> RLYRADSRPPDEIKRSGGLMPRGHNEYFDRGTQMNINLYDHARGTQTGFVRYDDGYVSTSLSLRSAHLAGQSILSGYSTYYIYVIATAPNMFNVNDVLGVYSPHPYEQEVSALGGIPYSQIYGWYRVNFGVIDERLHRNREYRDRYYRNLNIAPAEDGYRLAGFPPDHQAWREEPWIHHAPQGCG;> GDTCNEETQNLSTIYLREYQSKVKRQIFSDYQSEVDIYNRI;>APQTITELCSEYRNTQIYTINDKILSYTESMAGKREMVIITFKSGETFQVEVPGSQHIDSQKKAIERMKDTLRITYLTETKIDKLCVWNNKTPNSIAAISMKN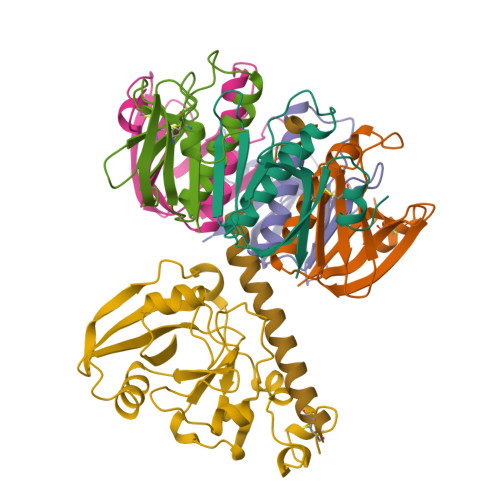[5x]> GSHMSGSKEEVPDNPPNEIYATAQQKLQDGNWRQAITQLEALDNRYPFGPYSQQVQLDLIYAYYKNADLPLAQAAIDRFIRLNPTHPNIDYVMYMRGLTNMALDDSALQGFFGVDRSDRDPQHARAAFSDFSKLVRGYPNSQYTTDATKRLVFLKDRLAKYEYSVAEYYTERG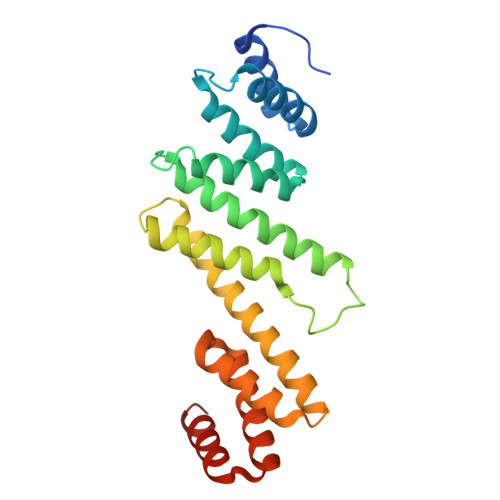AWVAVVNRVEGMLRDYPDTQATRDALPLMENAYRQMQMNAQAEKVAKIIAANSSNT>[3x]MLNPIVRKFQYGQHTVTLETGMMARQATAAVMVSMDDTAVFVTVVGQKKAKPGQDFFPLTVNYQERTYAAGRIPGSFFRREGRPSEGETLIARLIDRPIRPLFPEGFVNEVQVIATVVSVNPQVNPDIVAMIGASAALSLSGIPFNGPIGAARVGYINDQYVLNPTQDELKESKLDLVVAGTEAAVLMVESEAQLLSEDQMLGAVVFGHEQQQVVIQNINELVKEAGKPRWDWQPEPVNEALNARVAALAEARLSDAYRITDKQERYAQVDVIKSETIATLLAEDETLDENELGEILHAIEKNVVRSRVLAGEPRIDGREKDMIRGLDVRTGVLPRTHGSALFTRGETQALVTATLGTARDAQVLDELMGERTDTFLFHYNFPPYSVGETGMVGSPKRRE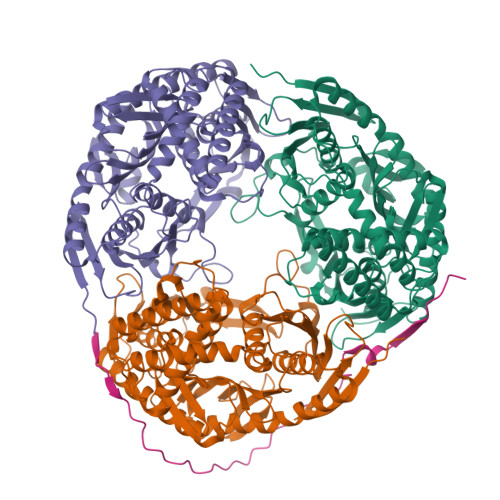IGHGRLAKRGVLAVMPDMDKFPYTVRVVSEITESNGSSSMASVCGASLALMDAGVPIKAAVAGIAMGLVKEGDNYVVLSDILGDEDHLGDMDFKVAGSRDGISALQMDIKIEGITKEIMQVALNQAKGARLHILGVMEQAINAPRGDIS;> NHATAPMTRAPAPEYVPEAPRHSDWQRPTFAFEGKGAAGGHTATHHASAAPARPQPVE>[2x]MQKLTVGLIGNPNSGKTTLFNQLTGARQRVGNWAGVTVERKEGIFATTDHQVTLVDLPGTYSLTTISSQ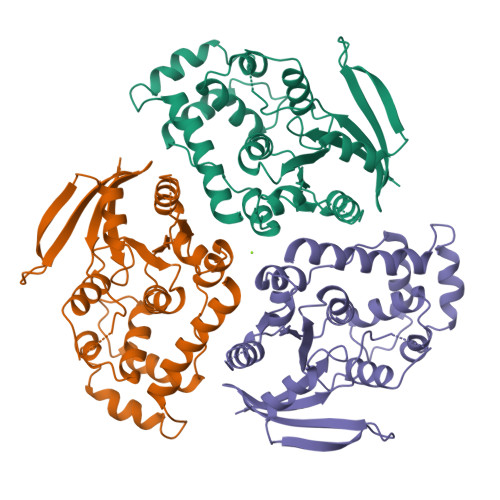TSLDEQIACHYILSGDADMLINVVDASNLERNLYLTLQLLELGIPCVVALNMLDIAEKQQVRIDIDALAARLGCPVIPLVSTRGRGIEALKIALDRHQANSDLELVHYPQPLLREADLLAQQMSAQIPPRQRRWLGLQMLEGDIYSRAYAGDAADKLDIALANLSDEIDDPALHIADARYQTIAAICDAVSNTLTAEP> MGSSHHHHHHSSGRENLYFQGPSNSDAAHAFWSTQPVPQTEDETEKIVFAGPMDEPKTVADIPEEPYPIASTFEWWTPNMEAADDIHAIYELLRDNYVEDDDS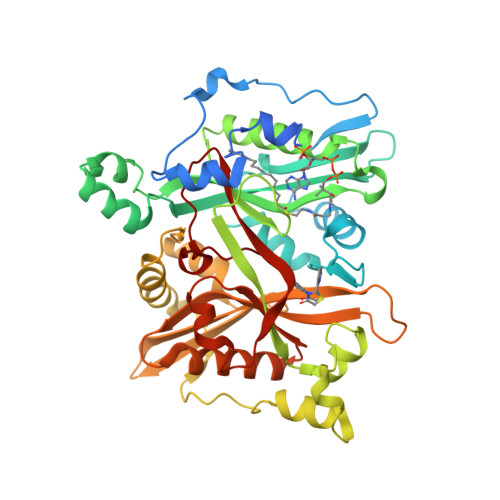MFRFNYSEEFLQWALCPPNYIPDWHVAVRRKADKKLLAFIAGVPVTLRMGTPKYMKVKAQEKGEGEEAAKYDEPRHICEINFLCVHKQLREKRLAPILIKEATRRVNRTNVWQAVYTAGVLLPTPYASGQYFHRSLNPEKLVEIRFSGIPAQYQKFQNPMAMLKRNYQLPSAPKNSGLREMKPSDVPQVRRILMNYLDSFDVGPVFSDAEISHYLLPRDGVVFTYVVENDKKVTDFFSFYRIPSTVIGNSNYNLLNAAYVHYYAATSIPLHQLILDLLIVAHSRGFDVCNMVEILDNRSFVEQLKFGAGDGHLRYYFYNWAYPKIKPSQVALVML> MENNGYKIILIGSSGVGKSSIVHQFLFNRKISNVSPTIGAAFASK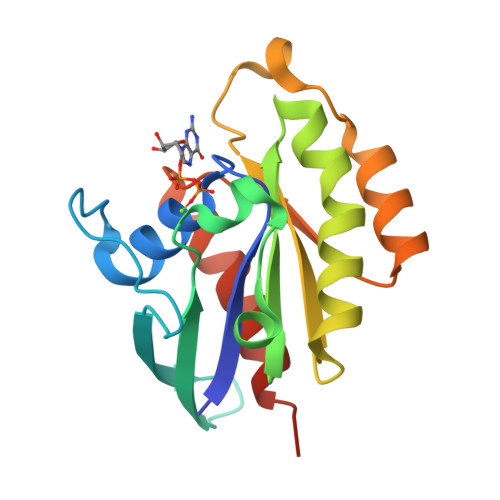QVIAKNGKTLKLNIWDTAGQERFRSITKMYYTNSLGCLVVFDVTDRESFDDVYYWINDLRINCHTTYYILVVANKIDIDKNNWRVSENEIKKFCRDNDCDYVFASSFESDTVNNLFGKMIDKMSEIKINPD> GSGNGGNGTEKADKKDGGKETITVMGPAEDLDDAQGAWLKTECEAFAKANPDFNIEFKYVTSSESDAKDVVTKDPKAAADVYMFANDQL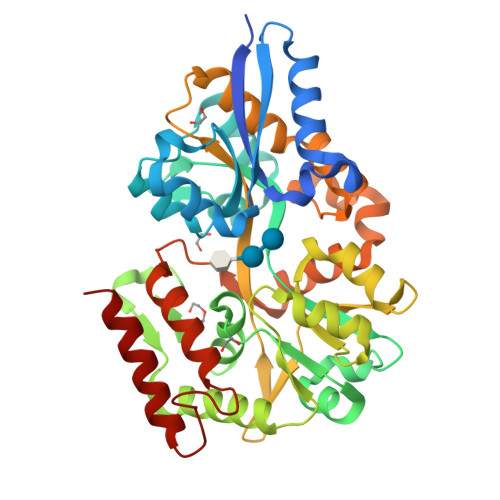EPLIKANAIAKLGGDTAEYVKSSNSEAMAATVTYDGDIYAVPYTSNTWFMYYDKRVFSEDDVKSLDTMLTKGKVSFPFDNGWYLNAFYAANGCTIFGDGTDKAAGYDFSGDKGTAVTNYIVDLFANPNFVMDNNEGSLGLAGLKDGSINAYFNGNWNYDKVKEALGEENVGVAALPTINIGGKDCQLKAFLGSKAIGVNPNCKNQEVAVKLAAFLGSEDAQLAHFKLRGQAPVNKDLATNEEVAADPVAAAMAKVSSDCSVAQPIIDMSGYWDAATPFGDAFQNGAEGQITKDNAAQKTEDFNTQLNDSLK>MAGRNWNASWIWGGQEESPRNEWRCFRGSFDAPASVEGPAMLHITADSRYVLFVNGEQVGRGPVRSWPKEQFYDSYDIGGQLRPGVRNTIAVLVLHFGVSNFYYLRGRGGLIAEIEADGRTLAATDAAWRTERLGGQRSNSPRMACQQGFGEVIDARELAEDWALPAFDDGGWAQARSIGPAGTAPWTSLVPRDIPFLTEEKLYPASIQSLSRVKAPKYAAALDLRNQMVPESVNHANPVSYCGYVATILTLETSGVVTLGFPTGVRGSGVWVDGVLQTEWTGVQPERYYSLNLAAGEHLVLVDITSSDHGGSSHFAIDSEAAFTLRSPAGDNGVPLATIGTFDQSEYIDHRPGRRMQTDHPDYRALPEAAPTAAALEAFASWVKPFEPSLYTEENVFGSNVWRTLAERRAVPRSVLNAILPVPEPGVLPVFEDGDCELVIDLGAERSGFIGFELEAPAGTIIDAYGVEYMREGYTQHTYGLDNTFRYICREGRQSYVSPVRRGFRYLFLTVRGNSAPVKLHEIYIR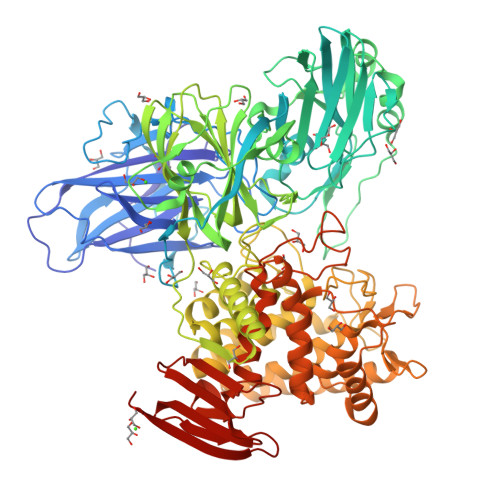QSTYPVAEQGSFRCSDALLNATWEISRHTTRLCMEDTFVDCPSYEQVFWVGDSRNEALVNYYVFGETEIVERCLNLVPGSADETPLYLDQVPSAWSSVIPNWTFFWILACREYAAHTGNEAFAARIWPAVKHTLTHYLEHIDDSGLLNMAGWNLLDWAPIDQPNEGIVTHQNLFLVKALRDSRALAAAAGATEEADAFAARADLLAETINAVLWDEEKRAYIDCIHADGRRSDVYSMQTQVVAYLCGVAQGEREAVIEGYLSSPPPAFVQIGSPFMSFFYYEALEKAGRQTLMLDDIRRNYGQMLRYDATTCWEMYPNFAENRSNPDMLTRSHCHAWSAAPGYFLGSSILGVKRGADGWRTVDIAPQPCDLTWAEGVVPLPQGGHIAVSWEFVSAGKLKLRIEAPEDIEVNVTLPEGIEGEVTQVKYMS[2x]> MALSKSMHARNRYKDKPPDFAYLASKYPDFKQHVQINLNGRVSLNFKDPEAVRALTCTLLREDFGLSIDIPLERLIPTVPLRLNYIHWVEDLIGHQDSDKSTLRRGIDIGTGASCIYPLLGATLNGWYFLATEVDDMCFNYAKKNVEQNNLSDLIKVVKVPQKTLLMDALKEESEIIYDFCMCNPPFFANQLEAKGVNSRNPRRPPPSSVNTGGITEIMAEGGELEFVKRIIHDSLQLKKRLRWYSCMLGKKCSLAPLKEELRIQGVPKVTYTEFCQGRTMRWALAWSFYD

METTL16 is the second m6A methyltransferase identified, and its known substrates include U6 snRNA and the human MAT2A mRNA that encodes for S-adenosylmethionine (SAM) synthetase (Pendleton et al., 2017). Here we describe the crystal structure of human METTL16 to reveal a methyltransferase domain furnished with an extra N-terminal module, which together form a deep-cut groove that is essential for RNA binding. Consistent with the SAM-dependent methyltransferase activity of METTL16, both structures reveal a Rossmann fold composed of a central seven-stranded β sheet (strands β3–β9) flanked by three α helices each (helices α4–α6 and α7–α9). In contrast, we show here that METTL16 is active as a monomer, and it contains a large deep-cut groove that can accommodate structured RNAs.

Two constructs (core, 1–291 aa; and ΔN, 40–291 aa) encompassing the methyltransferase domain (MTase) were expressed in E. coli and crystallized (Star Methods). First, and most striking, is the presence of an N-terminal module (1–78 aa) in the core structure that is appended to the α4 of the Rossmann fold and that consists of three helices (α1–α3) and two short β strands (β1 and β2). Taken together, our two structures reveal an architecture where the MTase domain is attached to a METTL16-specific N-terminal module that is essential for activity. Indeed, when mapped onto the METTL16-core structure, these reveal a positively charged cluster (K5, R10, R12, K14, K16, and R41) that forms the entrance of a wide deep-cut groove. With additional contributions from the N-terminal module (K47 and R74) and those from within the Rossmann fold (R82, R279, and R282), the groove runs all the way to the catalytic pocket containing the bound SAH. The residues K47 and R279 serve to constrict the space within this groove, while R74 overlooks the ridge that surrounds the SAH-binding pocket. The complexed byproduct of the SAM-dependent methylation reaction, S-adenosyl homocysteine (SAH), is coordinated by a hydrogen bond interaction network with the highly conserved amino acid residues R82, D108, G110, T111, S114, E133, Q162, N184, and R230. While 20 residues between Q191 and T212 are not visible in the ΔN structure, a much larger region (35 residues) between F187 and G223 lacks density in the core structure. The full-length METTL16 and the core domain versions were able to methylate this RNA (RNA6) at a specific adenosine residue (A17) within the nonamer UACAGAGAA motif. Strikingly, a combined mutant with all five residues converted to alanine (MUT1: K5A, R10A, R12A, K14A, and K16A) completely eliminated RNA methylation activity.>[3x]GSSGSSGMQIGKIIKVSGPLVMAENMSEACIQDMCLVGDLGVIGEIIEMRQDVASIQVYEETSGIGPGEPVRSTGEALSVELGPGIISQMFDGIQRPLDTFMEVTQSNFLGRGVQLPALDHEKQWWFEATIEEGTEVSAGDIIGYVDETKIIQHKIMVPNGIKGTVQKIESGSFTIDDPICVIETEQGLKELTMMQKWPVRRGRPIKQKLNPDVPMITGQRVIDTFFPVTKGGAAAVPGPFGAGKTVVQHQIAKWSDVDLVVYVGCGERGNEMTDVVNEFPELIDPNTGESLMERTVLIANTSNMPVAAREASIYTGITIAEYFRDMGYDVAIMADSTSRWAEALREMSGRLEEMPGDEGYPAYLGSRLAEYYERSGRVIALGSDQREGSITAISAVSPSGGDISEPVTQNTLRVVKVFWGLDSSLAQKRHFPSINWIQSYSLYSTEVGRYMDQILQQDWSDMVTEGMRILQEEEQLNEIVRLVGIDSLSDNDRLTLEVAKSIREDYLQQNAFDDVDTFTSREKQFNMLKVILTFGKEARKALSLGAYFNEIMEGTVAVRERISRSKYIPEEELAKISSINEEIKETIQLIVSEGGMTDD;>GSSGSSGMIKEYRTIKEVVGPLMAVEKVSGVKYEELIEVRMQNGEIRRGQVLEVQEDKAMVQIFEGTSGICLKNSSVRFLGHPLQLGVSEDMIGRVFDGLGRPKDNGPEILPEKYLDINGEVINPIARDYPDEFIQTGISAIDHLNTLVRGQKLPVFSGSGLPHKELAAQIARQATVLDSSDDFAVVFAAIGITFEEAEFFMEDFRQTGAIDRSVMFMNLANDPAIERIATPRMALTAAEYLAYEKGMHVLVIMTDMTNYAEALREISAARREVPGRRGYPGYLYTNLATLFERA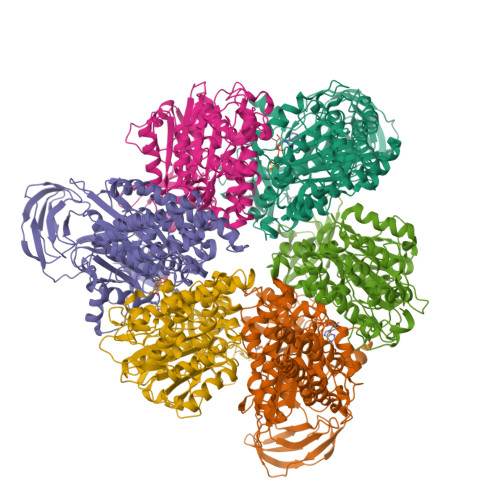GRIRGLKGSVTQIPILTMPEDDKTHPIPDLTGYITEGQIILTRELYKSGIQPPIDVLPSLSRLKDKGTGAGKTREDHAATMNQLFAAYAQGKQAKELAVVLGESALSDIDKIYAKFAERFENEYVNQGFYTNRTITETLDLGWELLAMLPRTELKRIKDDLLDKYLPEGK[3x]> GSFTSHQVAGHMYGKDKVGILQHPDGTVLKQLQPPPRGPRELEFYNMVYAADCFDGVLLELRKYLPKYYGIWSPPTAPNDLYLKLEDVTHKFNKPCIMDVKIGQKSYDPFASSEKIQQQVSKYPLMEEIGFLVLGMRVYHVHSDSYETENQHYGRSLTKETIKDGVSRFFHNGYCLRKD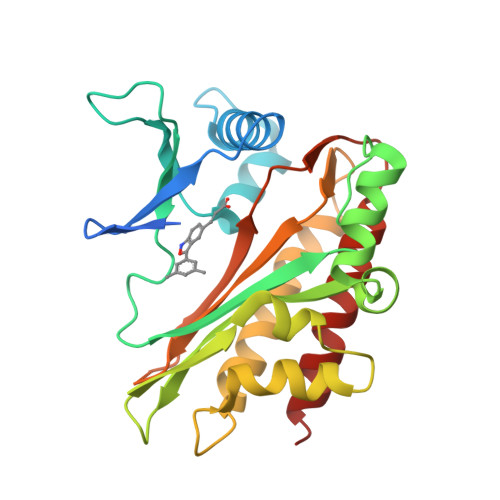AVAASIQKIEKILQWFENQKQLNFYASSLLFVYEGSSQGGSGGEVEVRMIDFAHVFPSNTIDEGYVYGLKHLISVLRSILDN>MFVFEDILKLDDRSIQLVLREVDTRDLALALKGASDELKEKIFKNMSKRAAALLKDELEYMGPV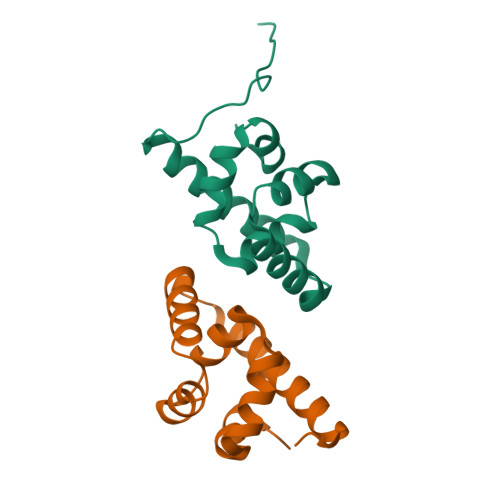RLKDVEEAQQKIINIIRRLEEAGEIVIARGGGEELIM[2x]1-METHYL-3-(N-PHENYLCARBAMIMIDOYL)UREA | C9 H12 N4 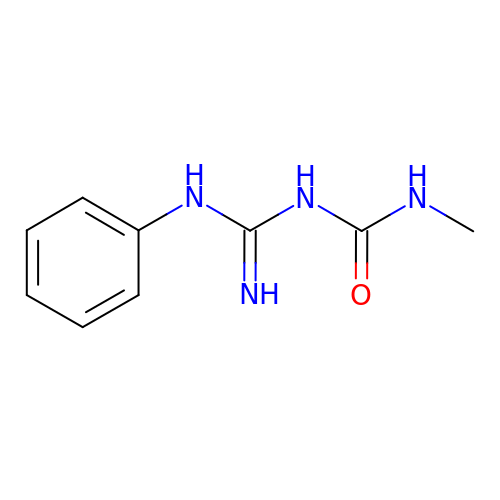O | BBCGZOVGNWCXHT-UHFFFAOYSA-N2-[(3-HYDROXY-2-METHYL-5-PHOSPHONOOXYMETHYL-PYRIDIN-4-YLMETHYLENE)-AMINO]-SUCCINIC 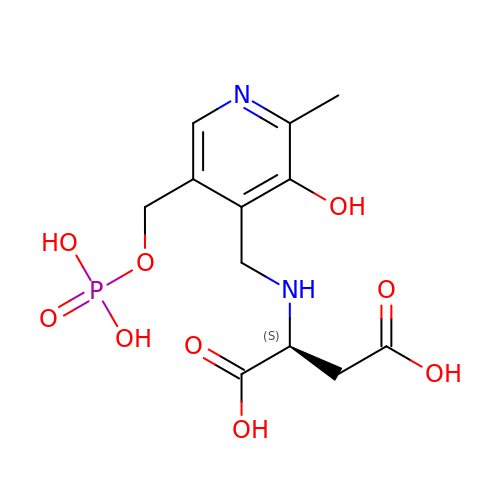ACID | C12 H17 N2 O9 P | UKHLSCZNRCHWTM-VIFPVBQESA-N> VPQKPKVSLNPPWNRIFKGENVTLTCNGNNFFEVSSTKWFHNGSLSEETNSSLNIVNAKFEDSGEYKCQHQ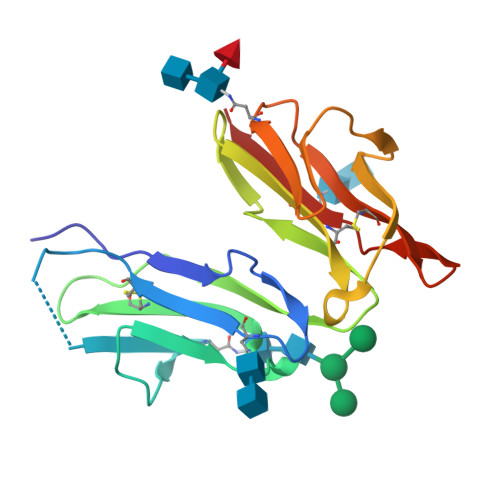QVNESEPVYLEVFSDWLLLQASAEVVMEGQPLFLRCHGWRNWDVYKVIYYKDGEALKYWYENHNISITNATVEDSGTYYCTGKVWQLDYESEPLNITVCKA>TKTGYINAAFRSSRNNEAYLFINDKYVLLDYAPGTSNDKVLYGPSFVRDGYKSLAKTIFGTYGIDCSFDTEYNEAFIFYENFCARIDYAPHSDKDKIISGPKKIADMFPFFKGTVFENGIDAAFRSTKGKEVYLFKGDKYARIDYLTNRLVQNIKSISDGFPCLRGTIFEAGMDSAFASHKTNEAYLFKGEYYARINFTPGSTNDIMGGVKKTLDYWPSLRGI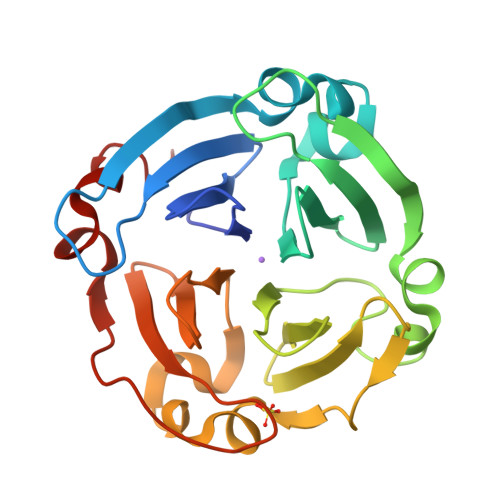IPLE[2x]> YNSGKLEEFVRGNLERECKEEKCSF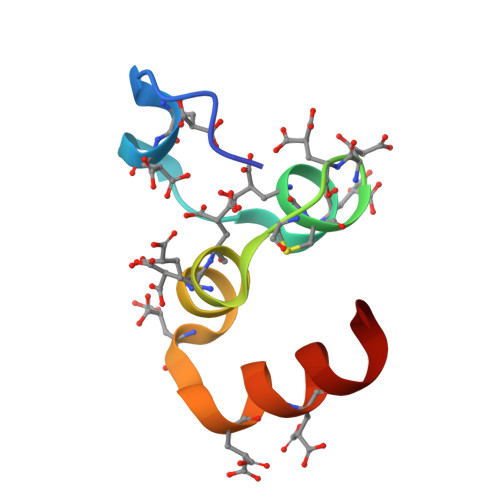EEAREVFENTEKTTEFWKQYV(1R,3R)-5-[(2E)-2-[(1R,3aS,7aR)-7a-methyl-1-[(2R)-6-oxidanyl-7-phenyl-6-(phenylmethyl)heptan-2-yl]-2,3,3a,5,6,7-hexahydro-1H-inden-4-ylidene]ethylidene]-2-methylidene-cyclohexane-1,3-diol | C39 H52 O3 | 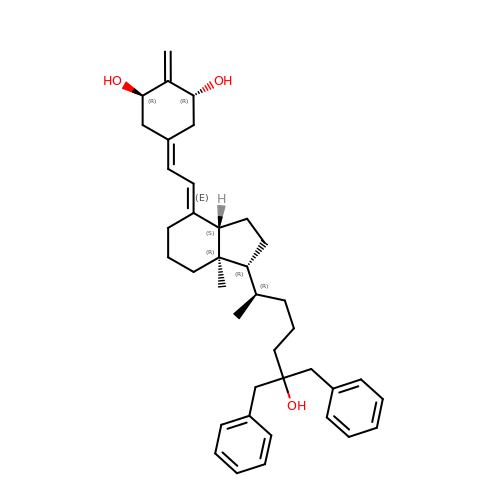RRDOSUMZWOEOPZ-BYWDIONYSA-N>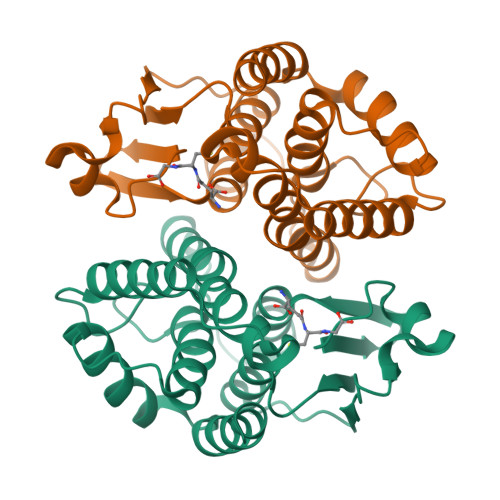 MDLYYRPGSAPCRSVLMTAKALGVEFDKKTIINTRAREQFTPEYLKINPQHTIPTLHDHGFALWESRAIMVYLVEKYGKDDKLFPKDVQKQALINQRLYFDMGTLYKSFSEYYYPQIFLKKPANEENYKKIEVAFEFLNTFLEGQTYSAGGDYSLADIAFLATVSTFDVAGFDFKRYANVARWYENAKKLTPGWEENWAGCQEFRKYFDN>CLRANDAPIVLLHGFTGWGREEMFGFKYWGGVRGDIEQWLNDNGYRTYTLAVGPLSSNWDRACEAYAQLVGGTVDYGAAHAAKHGHARFGRTYPGLLPELKRGGRIHIIAHSQGGQTARMLVSLLENGSQEEREYAKAHNVSLSPLFEGGHHFVLSVTTIATPHDGTTLVNMVDFTDRFFDLQKAVLEAAAVASNVPYTSQVYDFKLDQWGLRRQPGESFDHYFERLKRSPVWTSTDTARYDLS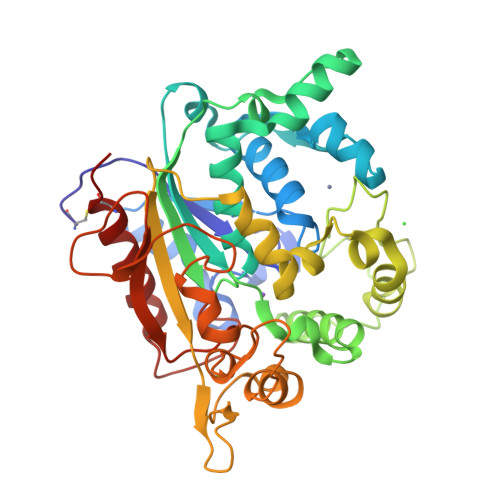VSGAEKLNQWVQASPNTYYLSFSTERTYRGALTGNHYPELGMNAFSAVVCAPFLGSYRNPTLGIDDRWLENDGIVNTVSMNGPKRGSSDRIVPYDGTLKKGVWNDMGTYNVDHLEIIGVDPNPSFDIRAFYLRLAEQLCSLQP[2x]2-TRIFLUOROMETHYL-5-METHYLENE-5H-PYRIMIDIN-4-YLIDENEAMINE | C6 H4 F3 N3 | 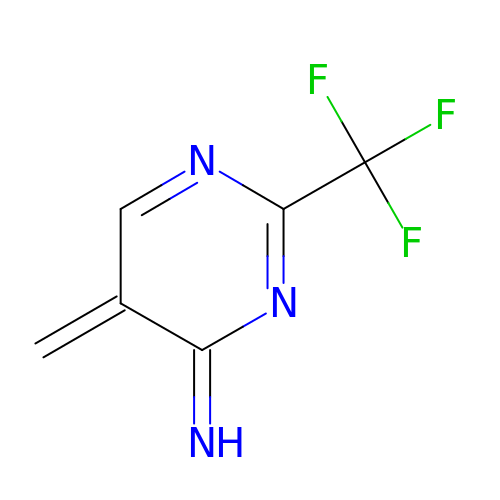YKFRUALXTUDSBW-UHFFFAOYSA-N> MSSQIRQNYSTEVEAAVNRLVNLYLRASYTYLSLGFYFDRDDVALEGVCHFFRELAEEKREGAERLLKMQNQRGGRALFQDLQKPSQDEWGTTLDAMKAAIVLEKSLNQALLDLHALGSAQADP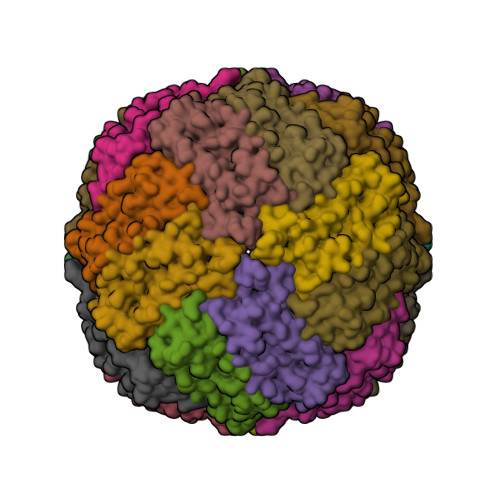HLCDFLESHFLDEEVKLIKKMGDHLTNIQRLVGSQAGLGEYLFERLTLKHD> QDN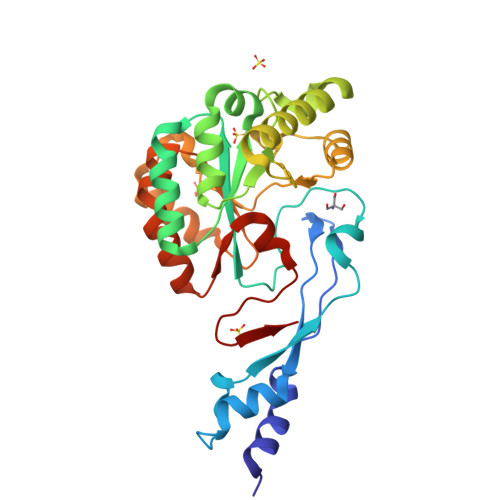LYEEIQKHAKQYEIAPQNAMIDKIWKATPGYNGRQVDMEASYNNMKKLKKFDQKHLEFKEVSPSVHLEDLSPAPIYRGHPNKKMVGLTINVAWGNEYLPRILEILKKHDVKATFFLEGRWVKENLRFAKMIVDANQEVGNHSYTHPNMKTLSSDEIRDQLQKTNRMIEAATNQKVRWFAPPSGSFRDEVVKIADDFQMGTIMWTVDTIDWKRPEPDVLLQRVMRKIHPGAIVLMHPTSSTTEALDTMITKLKEQGYKVGNITELLDEKRVDLEHHHHHH>GAMGDGEMLLIINEYGSPLGLTALPDKEHGGGLLVQHVEPGSRAERGRLRRDDRILEINGIKLIGLTESQVQEQLRRALESSELRVRVLRGDRNGGGSGSGGG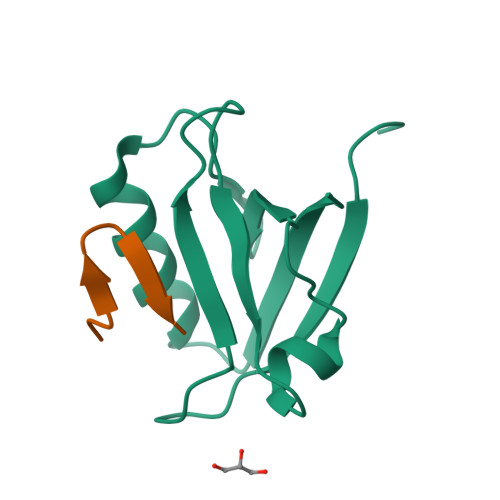GSGGSGVKDGVLHL[4x]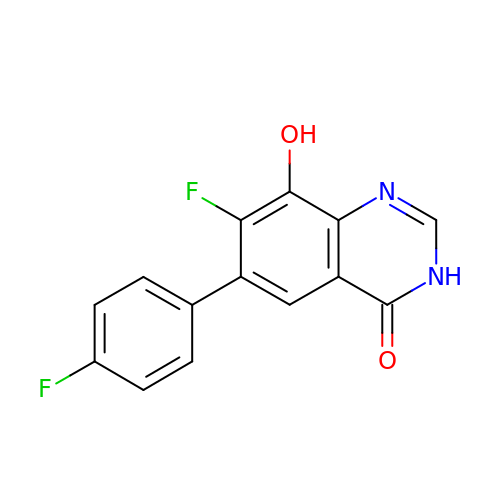7-fluoranyl-6-(4-fluorophenyl)-8-oxidanyl-3~{H}-quinazolin-4-one | C14 H8 F2 N2 O2 | UPRNZWUAFGVMOP-UHFFFAOYSA-N>MDENHSDSNLPEGTEPAGRPAPRTDMTVNEMREWLRNWVANATGQSADAIDESTPMVELGLSSRDAVAMASDIEDLTGVTLTATVAFRHPTIESLATVIIEGEPEPEPYDEDEDWSRTRDVEDIAIVGVATRFPGDLNTPDEMWEALLEGKDCVTDLPEDRWTEFLDEPRIAERVKKARTRGGYLTDIKGFDSEFFALSKMEADNIDPQQRMALELTWEALEHARIPASSLRGESVGVYIGSSTNDYSFLAMSDPSIAHPYAITGTASSIIANRVSYFYDFRGPSVAVDTACSSSLVATHQGVQALRAGEADVAIVGGVNALVTPLVTVGFDEVGGVLAPDGRIKSFSSDADGYARSEGGGMLVLKRISDARRDGDQILAVIAGSAVNHDGRSNGLLAPNPDAQAEVLRKAYKDAGINPRDVDYIEAHGTGTILGDPIEADALGRIVGKGRPADKPALLGAVKSNLGHLESAAGAASLAKMTLALANDKLPPSINYAGPNPYIDFEKERLKVNDTVSDWPRYSGKAIAGVSGFGFGGANAHVVMREVLAGDLVEPEPEPEPEAKPEKSEADAVYVGGVRMDEYGEFIDEDEPAEGGDAYPSYDEDSYELPGITEAAQRLLEQAREELEAKEAEEPTKQLVPLAVSAFLTSRKRQAAAELADWIDSPEGRASSLESIGRSLSRRNHGRSRAVVLAHDHDEAIKGLRALAEGKQHPSVLSADGPVTNGPVWVLAGFGAQHRKMGKSLYLRNEVFAEWINKVDALIQDERGYSILELILDDNVDYTDATCEYPIEVVQLVIFAIQIALGELLRHHGAKPAAVVGQSLGEAAASYFAGGLSLADATRTICSRSHLMGEGEAMLFGEYIRLMALVEYSADEIKTVFSDYPDLEVCVYAAPTQTVIGGPPDQVDAIIARAESEGKFARKFQTKGASHTQQMDPLLGELAAELQGIEPKPLTTGYFSTVHEGTFIRPGSAPIHDVDYWKKGLRHSVYFTQGIRNAVDNGHTTFLELAPNPVALMQVGLTTASAGLHDAQLIATLARKQDEVESMISAMAQLYVHGHDLDFRTLFPRRSKGLAGALDFANIPPTRFKRKEHWLPAHFTGDSSAVMPGNHVATPDGRHVWEFVPRGKTDLAALVKAAAAQVLPDAKLAAFEQRAVPADNARLVTTLTRHPGGATVQVHARVEESFTLVYDAIVARANGAGVTALPVAVGAGVAVSGDVAGEGAGASVIEDDEPDAEILQDNLTAGAGMGADFQKWDPNSGETIGQRLGTIVGAAMGYEPEDLPWEVPLIELGLDSLMAVRIKNRVEYDFDLPPIQLTAVRDANLYNVEELIRYAIEHRDEVEQIAESQKGKTAEEIAAEQSELLGGASTVAELEAKLAEAGHPLAAKDSEDSENSEDNAAGAAAAAEASAVEGLEIPPPPTDPTGPGGAPIPPPPSDPSGPAQAASATDAPAGTVNKATAAAAAAKVLTQEAVTEALGADVPPRDAAERVTFATWAIVTGKSPGGIFNELPTVSEETAKKMAERLSERAEGTITVEDVLGAKTIEGLATIVREQLEEGVVDGFVRTLRPPKEGSNAVPLFVFHPAGGSTVVYEPLMKRLPADVPVYGLERVEGSIE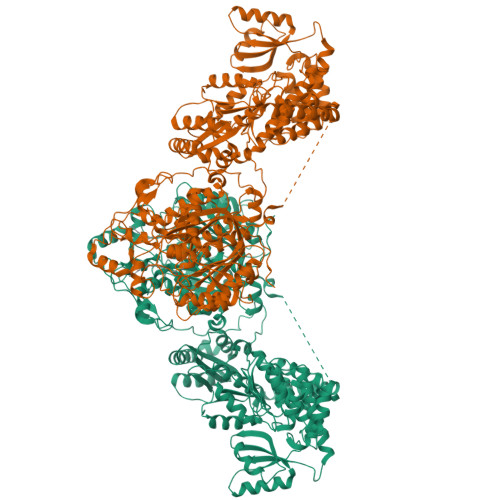ERAAEYVPKLLEMHKGPFVLAGWSLGGALAYACAIGLKQSGADVRFVGLIDTVLPGEPIDQSKEGMRARWDRYARFAERTFNVEIPAIPYEELEKLDDEGQVKYVLEIVKESGVQIPGGIIEHQRTSYLDNRALDTVDIKPYDGHVTLYMADRYHDDAIVFEPAYATRKPDGGWGSFVSDLEVVHIGGEHIQAIDEPYIAKVGAHMSEALNRIEAQASKEDGAKSKSTSENLYFQ[2x]> MAGGA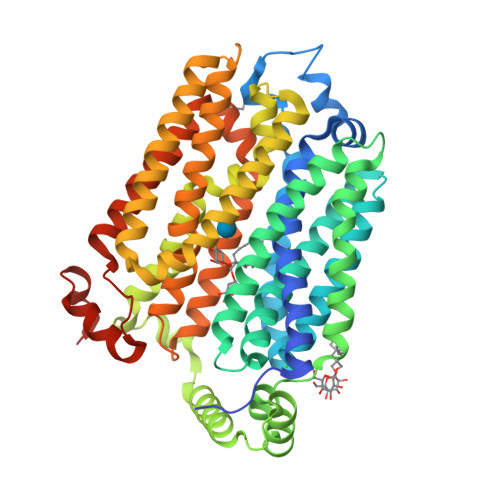FVSEGGGGGRSYEGGVTAFVIMTCIVAAMGGLLFGYDLGISGGVTSMEEFLTKFFPQVESQMKKAKHDTAYCKFDNQMLQLFTSSLYLAALVASFMASVITRKHGRKVSMFIGGLAFLIGALFNAFAVNVSMLIIGRLLLGVGVGFANQSTPVYLSQMAPAKIRGALNIGFQMAITIGILVANLINYGTSKMAQHGWRVSLGLAAVPAVVMVIGSFILPDTPNSMLERGKNEEAKQMLKKIRGADNVDHEFQDLIDAVEAAKKVENPWKNIMESKYRPALIFCSAIPFFQQITGINVIMFYAPVLFKTLGFGDDAALMSAVITGVVNMLSTFVSIYAVNRYGRRLLFLEGGIQMFICQLLVGSFIGARFGTSGTGTLTPATADWILAFICVYVAGFAWSWGPLGWLVPSEICPLEIRPAGQAINVSVNMFFTFLIGQFFLTMLCHMKFGLFYFFASMVAIMTVFIYFLLPETKGVPIEEMGRVWKQHWFWKKYIPEDAIIGGHDDNNTN> GSMADEATRRVVSEIPV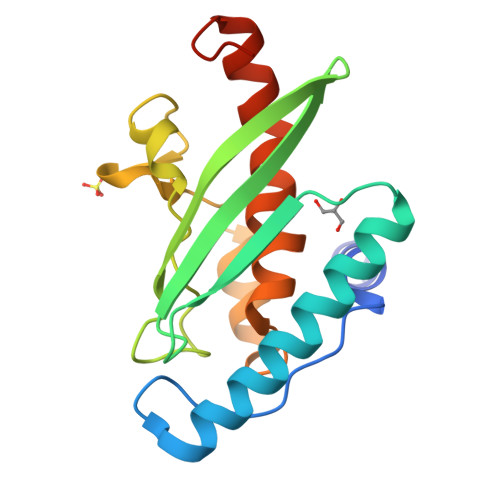LKTNAGPRDRELWVQRLKEEYQSLIRYVENNKNADNDWFRLESNKEGTRWFGKCWYIHDLLKYEFDIEFDIPITYPTTAPEIAVPELDGKTAAMYRGGKIELTDHFKPLWARNVPKFGLAHLMALGLGPWLAVEIPDLIQKGVIHHKEKCNQ> ATDVATVVSQAKAQMKEAYYTYSHTVTETGQFPDIKDVYAAYNKAKQAYANAVAVVNKAGGAKKDAYLADLQAIYETYVFKANPKSGEARVATYIDAYNYATKLDKMRQELKAAVDAKDLKKAEELYHKISYELKTRTVILDRVYGQSTRELLRSTFKADAQALRDRLIYDITVAMKAREAQDAVKAGNLDKAKAALDQVNQYVSKVTDAFKAELQKAAQDAKAAYEAALTPKVESVSAIDSTSFKVTFTKPVDKATAIPKNFSITLKGTETKLYPKSVEVSESGLTATVTLYDTLVDGKTYTVVTSGLKDTAGKEFETSTNEFTYNKPVPASITFNFNKLPEDSAVDLTKYVTVKDAAGNVIKSGFELEFTSSEKLTQGKFINTTGKKSVIVNATVKGTNVTTGNVILAVEDEKAAEVSELKLTKDNKEVVTLYANGNAFDKDGNQISSGTLTLTAKFKDQYGNELTGKVAGTDYTFESLNPEVLVVAPDGSVTPIVPGTALVKVKYGEVTKTIPVTVKANPVLETIAVDSTGVSVAKGQKATFKVTLKDQYGNKFTGNVNVTSDKTETATVSVSNSGIGQSEYTVTVNGVAEGSTTITIKSGTKEVKVPVNVVAGGPVANYQIKVLDDGKIDKSATESPANNDVQLKVYAVDANGNIVGDITNDVTITSEATDTNGVIVNASKSTANGDTVYVITDNGSKKVGKETLTVKLGTVT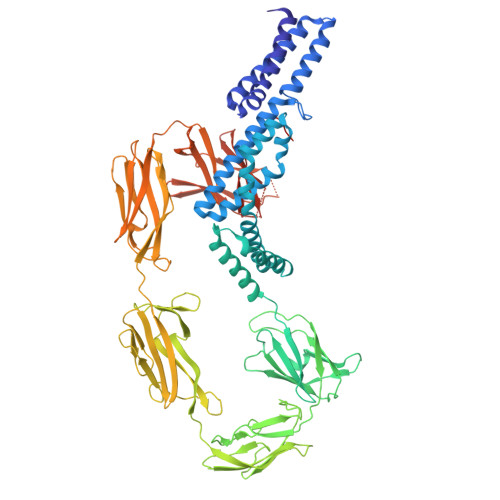LGTVDVEVIDTTLKATVVTKKADLIELDAADNGDALAKLLANL> LILNLRGGAFVSNTQITMADKQKKFINEIQEGDLVRSYSITDETFQQNAVTSIVKHEADQLCQINFGKQHVVCTVNHRFYDPESKLWKSV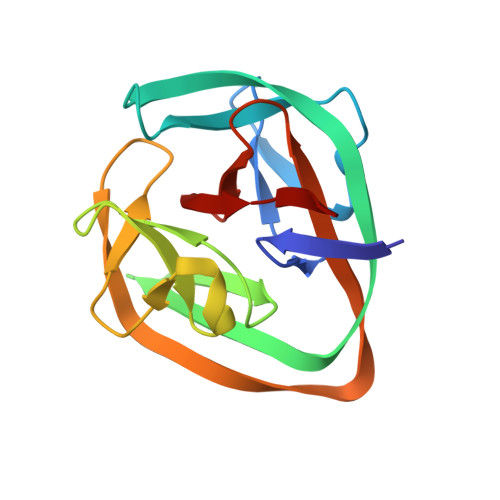CPHPGSGISFLKKYDYLLSEEGEKLQITEIKTFTTKQPVFIYHIQVENNHNFFANGVLAHAMQVS>[2x]MSNQYGDKNLKIFSLNSNPELAKEIADIVGVQLGKCSVTRF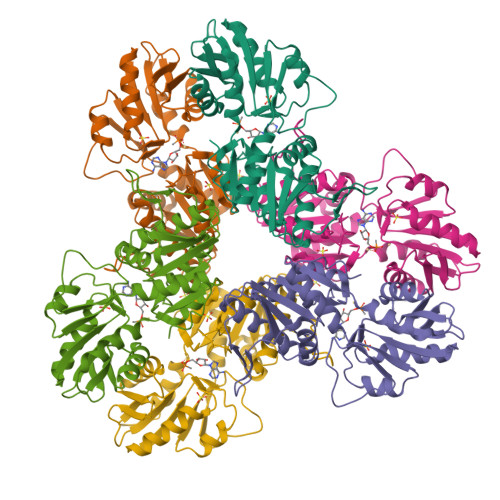SDGEVQINIEESIRGCDCYIIQSTSDPVNEHIMELLIMVDALKRASAKTINIVIPYYGYARQDRKARSREPITAKLFANLLETAGATRVIALDLHAPQIQGFFDIPIDHLMGVPILGEYFEGKNLEDIVIVSPDHGGVTRARKLADRLKAPIAIIDKRRPRPNVAEVMNIVGNIEGKTAILIDDIIDTAGTITLAANALVENGAKEVYACCTHPVLSGPAVERINNSTIKELVVTNSIKLPEEKKIERFKQLSVGPLLAEAIIRVHEQQSVSYLFS> MSFTPANRAYPYTRLRRNRRDDFSRRLVRENVLTVDDLILPVFVLDGVNQRESIPSMPGVERLSIDQLLIEAEEWVAL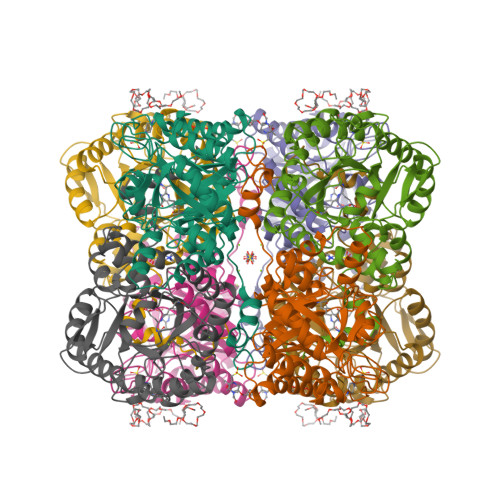GIPALALFPVTPVEKKSLDAAEAYNPEGIAQRATRALRERFPELGIITDVALDPFTTHGQDGILDDDGYVLNDVSIDVLVRQALSHAEAGAQVVAPSDMMDGRIGAIREALESAGHTNVRIMAYSAKYASAYYGPFRDAVGSASNLGKGNKATYQMDPANSDEALHEVAADLAEGADMVMVKPGMPYLDIVRRVKDEFRAPTFVYQVSGEYAMHMGAIQNGWLAESVILESLTAFKRAGADGILTYFAKQAAEQLRRGR>HHHHHHLESTSLYKKAGMATANGAVENGQPDRKPPALPRPIRNLEVKFTKIFINNEWHESKSGKKFATCNPSTREQICEVEEGDKPDVDKAVEAAQVAFQRGSPWRRLDALSRGRLLHQLADLVERDRATLAALETMDTGKPFLHAFFIDLEGCIRTLRYFAGWADKIQGKTIPTDDNVVCFTRHEPIGVCGAITPWNFPLLMLVWKLAPALCCGNTMVLKPAEQTPLTALYLGSLIKEAGFPPGVVNIVPGFGPTVGAAISSHPQINKIAFTGSTEVGKLVKEAASRSNLKRVTLELGGKNPCIVCADADLDLAVECAHQGVFFNQGQCCTAASRVFVEEQVYSEFVRRSVEYAKKRPVGDPFDVKTEQGPQIDQKQFDKILELIESGKKEGAKLECGGSAMEDKGLFIKPTVFSEVTDNMRIAKEEIFGPVQPILKFKSIEEVIKRANSTDYGLTAAVFTKNLDKALKLASALESGTVWINCYNALYAQAPFGGFKMSGNGRELGEYALAEYTEVKTVTIKLGDKNP[2x]

The human aldehyde dehydrogenase (ALDH) superfamily comprises 19 enzyme isoforms catalyzing the NAD(P)-dependent irreversible oxidation of aldehydes to their corresponding carboxylic acids. Cytosolic ALDH1A enzymes, and specifically the ALDH1A3 isoform, are good markers of cancer stem cells and have been implicated in carcinogenesis, chemoresistance and relapse. As previously observed in other members of the enzyme superfamily, each ALDH1A3 subunit is composed of three structural domains: a catalytic domain, a cofactor-binding domain and an oligomerization domain. At the intersection of the substrate- and cofactor-binding pockets sits a strictly conserved cysteine residue (Cys302, ALDH2 numbering), which is essential for catalysis, acting as the active-site nucleophile.

The ALDH1A3 apo structure at 2.29-Å resolution shows a few electron density blobs inside the substrate-binding pocket near the catalytic Cys314 in both monomers. These electron densities could not be modeled with any of the molecules present in the crystallization cocktail. A PEG molecule can also be seen within the substrate-binding pocket in both subunits of the crystal ALDH1A3 apo structure. All crystal structures contain a homodimer in the asymmetric unit (left). The cofactor-binding domain contains a non-canonical Rossmann-fold motif, slightly different from that found in other NAD(P)+-dependent enzymes. The three crystal structures described in this work do not present remarkable conformational changes among them and share the same disordered areas. The volume of the pocket in the cofactor-binding domain is 444, 439 and 411 Å3 for the apo form, the ALDH1A3-NAD+ and the ALDH1A3-ATP complexes, whereas the volumes of the substrate-binding pockets are 231, 220 and 208 Å3 for the same forms, respectively.ERGIC-53 transports certain subsets of newly synthesized secretory proteins and membrane proteins from the endoplasmic reticulum to the Golgi apparatus. MCFD2 is a small protein composed of an EF-hand domain with two Ca2+ binding sites, and functions as a binding partner of ERGIC-53 in a Ca2+-dependent manner. From the amino acid sequence, ERGIC-53 is predicted to be a single-pass transmembrane protein that consists of a luminal carbohydrate recognition domain (CRD), a long stalk domain, a transmembrane (TM) helix and a short cytoplasmic tail (CT). Here we present cryo-EM structures of full-length ERGIC-53 in complex with its functional partner MCFD2. These structures reveal that ERGIC-53 exists as a homotetramer, not a homohexamer as previously suggested, and comprises a four-leaf clover-like head and a long stalk composed of three sets of four-helix coiled-coil followed by a transmembrane domain.

The two different structures of the head region suggest its conformational variability. In component IIhead, two CRD dimers rotate along a vertical axis (i.e., nearly parallel to the central coiled-coil) in opposite directions (referred to as twisting motion) (right). In the superposition of substate structures C and D, S-H1 and MCFD2 in the upper layers and those in the lower layers rotate by 2.5˚ and 1.9˚, respectively, breaking the C2 symmetry of the head region. These rotations seem to be ascribed to the flexible loops between the CRD and S-H1 and between S-H1 and S-H2. Thus, the two loops within the head region likely generate the plasticity of the head region, allowing the CRD-MCFD2 complex to fluctuate continuously in the tetrameric structure.

>[4x]MAGSRQRGLRARVRPLFCALLLSLGRFVRGDGVGGDPAVALPHRRFEYKYSFKGPHLVQSDGTVPFWAHAGNAIPSSDQIRVAPSLKSQRGSVWTKTKAAFENWEVEVTFRVTGRGRIGADGLAIWYAENQGLEGPVFGSADLWNGVGIFFDSFDNDGKKNNPAIVIIGNNGQIHYDHQNDGASQALASCQRDFRNKPYPVRAKITYYQNTLTVMINNGFTPDKNDYEFCAKVENMIIPAQGHFGISAATGGLADDHDVLSFLTFQLTEPGKEPPTPDKEISEKEKEKYQEEFEHFQQELDKKKEEFQKGHPDLQGQPAEEIFESVGDRELRQVFEGQNRIHLEIKQLNRQLDMILDEQRRYVSSLTEEISKRGAGMPGQHGQITQQELDTVVKTQHEILRQVNEMKNSMSETVRLVSGMQHPGSAGGVYETTQHFIDIKEHLHIVKRDIDNLVQRNMPSNEKPKCPELPPFPSCLSTVHFIIFVVVQTVLFIGYIMYRSQQEAAAKKFFGVAMPGAEDDVV;>[4x]GSHMEEPAASFSQPGSMGLDKNTVHDQEHIMEHLEGVINKPEAEMSPQELQLHYFKMHDYDGNNLLDGLELSTAITHVHKEEGSEQAPLMSEDELINIIDGVLRDDDKNNDGYIDYAEFAKSLQ> VALSRTQVCGILREELFQGDAFHQSDTHIFIIMGASGDLAKKKIYPTIWWLFRDGLLPENTFIVGYARSRLTVADIRKQSEPFFKATPEEKLKLEDFFARNSYVAGQYDDAASYQRLNSHMNALHLGSQANRLFYLALPPTVYEAVTKNIHESCMSQIGWNRIIVEKPFGRDLQSSDRLSNHISSLFREDQIYRIDHYLGKEMVQNLMVLRFANRIFGPIWNRDNIACVILTFKEPFGTEGRGGYFDEFGIIRDVMQNHLLQMLCLVAMEKPASTNSDDVRDEKVKVLKCISEVQANNVVLGQYVGNPDGEGEATKGYLDDPTVPRGSTTATFAAVVLYVENERWDGVPFILRCGKALNERKAEVRLQFHDVAGDIFHQQCKRNELVIRVQPNEAVYTKMMTKKPGMFFNPEESELDLTYGNRYKNVKLPDAYERLILDVFCGSQMHFVRSDELREAWRIFTPLLHQIELEKPKPIPYIYGSRGPTEADELMKRVGFQYEG;> ALSRTQVCGILREELFQGDAFHQSDTHIFIIMGASGDLAKKKIYPTIWWLFRDGLLPENTFIVGYARSRLTVADIRKQSEPFFKATPEEKLKLEDFFARNSYVAGQYDDAASYQRLNSHMNALHLGSQANRLFYLALPPTVYEAVTKNIHESCMSQIGWNRIIVEKPFGRDLQSSDRLSNHISSLFREDQIYRIDHYLGKEMVQNLMVLRFANRIFGPIWNRDNIACVILTFKEPFGTEGRGGYFDEFGIIRDVMQNHLLQMLCLVAMEKPASTNSDDVRDEKVKVLKCISEVQANNVVLGQYVGNPDGEGEATKGYLDDPTVPRGSTTATFAAVVLYVENERWDGVPFILRCGKALNERKAEVRLQFHDVAGDIFHQQCKRNELVIRVQPNEAVYTKMMTKKPGMFFNPEESELDLTYGNRYKNVKLPDAYERLILDVFCGSQMHFVRSDELREAWRIFTPLLHQIELEKPKPIPYIYGSRGPTEADELMKRVGFQY;>LSRTQVCGILREELFQGDAFHQSDTHIFIIMGASGDLAKKKIYPTIWWLFRDGLLPENTFIVGYARSRLTVADIRKQSEPFFKATPEEKLKLEDFFARNSYVAGQYDDAASYQRLNSHMNALHLGSQANRLFYLALPPTVYEAVTKNIHESCMSQIGWNRIIVEKPFGRDLQSSDRLSNHISSLFREDQIYRIDHYLGKEMVQNLMVLRFANRIFGPIWNRDNIACVILTFKEPFGTEGRGGYFDEFGIIRDVMQNHLLQMLCLVAMEKPASTNSDDVRDEKVKVLKCISEVQANNVVLGQYVGNPDGEGEATKGYLDDPTVPRGSTTATFAAVVLYVENERWDGVPFILRCGKALNERKAEVRLQFHDVAGDIFHQQCKRNELVIRVQPNEAVYTKMMTKKPGMFFNPEESELDLTYGNRYKNVKLPDAYERLILDVFCGSQMHFVRSDELREAWRIFTPLLHQIELEKPKPIPYIYGSRGPTEADELMKRVGFQY[2x];>[2x]VALSRTQVCGILREELFQGDAFHQSDTHIFIIMGASGDLAKKKIYPTIWWLFRDGLLPENTFIVGYARSRLTVADIRKQSEPFFKATPEEKLKLEDFFARNSYVAGQYDDAASYQRLNSHMNALHLGSQANRLFYLALPPTVYEAVTKNIHESCMSQIGWNRIIVEKPFGRDLQSSDRLSNHISSLFREDQIYRIDHYLGKEMVQNLMVLRFANRIFGPIWNRDNIACVILTFKEPFGTEGRGGYFDEFGIIRDVMQNHLLQMLCLVAMEKPASTNSDDVRDEKVKVLKCISEVQANNVVLGQYVGNPDGEGEATKGYLDDPTVPRGSTTATFAAVVLYVENERWDGVPFILRCGKALNERKAEVRLQFHDVAGDIFHQQCKRNELVIRVQPNEAVYTKMMTKKPGMFFNPEESELDLTYGNRYKNVKLPDAYERLILDVFCGSQMHFVRSDELREAWRIFTPLLHQIELEKPKPIPYIYGSRGPTEADELMKRVGFQY;> VALSRTQVCGILREELFQGDAFHQSDTHIFIIMGASGDLAKKKIYPTIWWLFRDGLLPENTFIVGYARSRLTVADIRKQSEPFFKATPEEKLKLEDFFARNSYVAGQYDDAASYQRLNSHMNALHLGSQANRLFYLALPPTVYEAVTKNIHESCMSQIGWNRIIVEKPFGRDLQSSDRLSNHISSLFREDQIYRIDHYLGKEMVQNLMVLRFANRIFGPIWNRDNIACVILTFKEPFGTEGRGGYFDEFGIIRDVMQNHLLQMLCLVAMEKPASTNSDDVRDEKVKVLKCISEVQANNVVLGQYVGNPDGEGEATKGYLDDPTVPRGSTTATFAAVVLYVENERWDGVPFILRCGKALNERKAEVRLQFHDVAGDIFHQQCKRNELVIRVQPNEAVYTKMMTKKPGMFFNPEESELDLTYGNRYKNVKLPDAYERLILDVFCGSQMHFVRSDELREAWRIFTPLLHQIELEKPKPIPYIYGSRGPTEADELMKRVGFQYE;> SRTQVCGILREELFQGDAFHQSDTHIFIIMGASGDLAKKKIYPTIWWLFRDGLLPENTFIVGYARSRLTVADIRKQSEPFFKATPEEKLKLEDFFARNSYVAGQYDDAASYQRLNSHMNALHLGSQANRLFYLALPPTVYEAVTKNIHESCMSQIGWNRIIVEKPFGRDLQSSDRLSNHISSLFREDQIYRIDHYLGKEMVQNLMVLRFANRIFGPIWNRDNIACVILTFKEPFGTEGRGGYFDEFGIIRDVMQNHLLQMLCLVAMEKPASTNSDDVRDEKVKVLKCISEVQANNVVLGQYVGNPDGEGEATKGYLDDPTVPRGSTTATFAAVVLYVENERWDGVPFILRCGKALNERKAEVRLQFHDVAGDIFHQQCKRNELVIRVQPNEAVYTKMMTKKPGMFFNPEESELDLTYGNRYKNVKLPDAYERLILDVFCGSQMHFVRSDELREAWRIFTPLLHQIELEKPKPIPYIYGSRGPTEADELMKRVGFQY

Glucose-6-phosphate dehydrogenase (G6PD) catalyzes the first and rate-limiting reaction in the PPP; the oxidation of glucose-6-phosphate (G6P) to 6-phosphogluconolactone with concomitant reduction of nicotinamide adenine dinucleotide phosphate (NADP+) to NADPH. G6PD is a major source of cellular NADPH and has a primary role in controlling the metabolic flux through the PPP. G6PD is catalytically active as a homodimer or homotetramer. Each monomer has one G6P binding site (i.e., the catalytic site) and can bind two NADP+ molecules; one is close to the G6P binding site, and the other is the structural NADP+ binding site.

To elucidate the molecular mechanism of G6PD inactivation by KAT9- and CBP-dependent K403 acetylation, we determined the crystal structure of AcK403 G6PD. The protein crystallized in the P1 space group, with eight monomers within the asymmetric unit, and the structure was determined at 2.28 Å resolution. That said, the structure of AcK403 included an α helix at the N-terminus (residues R9–Q22, hereafter referred to as αa’) that has not been observed in other crystal structures of human G6PD. Lysine 403-acetylated G6PD was crystallized without structural or catalytic NADP+, and a close examination of the structure revealed acetylation-dependent conformational changes at the dimer interface and the substrate binding site. In non-acetylated G6PD, positively charged K403 and R370 interact with the phosphate groups of NADP+. Following K403 acetylation, the acetylated residue adopts a different conformation that is stabilized by electrostatic interaction with R370, excluding the structural NADP+ from its binding site. This minor conformational change in the structural NADP+ binding site was accompanied by distortion of the β-sheet at the dimer interface (mainly βN) and unwinding of the short αl helix. First, the newly formed loop (formerly αl) reshaped the dimer interface, in line with the observed differences in the dimeric structure. Third, in AcK403 G6PD, K205 was rotated by ~180° relative to its position in WT G6PD, and held in position by electrostatic interaction with D443. This conformational change was accompanied by the unwinding of helix αf’, the disposition of helix αf away from the substrate binding site, and the reorientation of functionally important residues such as Y202, and H201, that together rendered the enzyme inactive. In summary, K403 acetylation-dependent conformational changes in the NADP+ binding site reshaped the dimer interface and propagated to the substrate binding site via partial unwinding of helices αl and αf’, disposition of helix αf, and deformation of the G6P binding site.>MASTVSNTSKLEKPVSLIWGCELNEQNKTFEFKVEDDEEKCEHQLALRTVCLGDKAKDEFHIVEIVTQEEGAEKSVPIATLKPSILPMATMVGIELTPPVTFRLKAGSGPLYISGQHVAMEEDYSWAEEEDEGEAEGEEEEEEEEDQESPPKAVKRPAATKKAGQAKKKLDKEDESSEEDSPTKKGKGAGRGRKPAAKK[5x]

In Xenopus eggs, NPM2 replaces sperm protamines with core histones upon fertilization, thereby promoting nucleosome assembly on sperm DNA Laskey et al., 1978; Philpott et al., 1991; Ohsumi and Katagiri, 1991. NPM2 can also extract out somatic linker histones from chromatin Dimitrov and Wolffe, 1996; Ramos et al., 2005; Bañuelos et al., 2007. The acidic tracts in the C-terminal tail of NPM2 binds H2A-H2B, histone octamers, and the linker histone H5 Platonova et al., 2011; Ramos et al., 2010; Taneva et al., 2009, while poly-glutamylation and hyperphosphorylation of NPM2 promote its substrate sequestration ; Lorton et al., 2023. Our cryo-EM structure strongly suggests that the NPM2 binds to H1.8 as a homo-pentamer.

By further analyzing our cryo-EM structure representing the H1.8-bound state of NPM2, we identified two structural variants, classified as open and closed forms. The major structural differences between the two forms are found at C-terminal and N-terminal segments of NPM2 core and at the A1 loop. In the open form, however, the C-terminal portion of β8 is bent outward to the rim. Along with this β8 bending, C-terminal segment, N-terminal segment, and A1 loop are also positioned outward in the open form. The bending is critical in forming the open-form NPM2 structures and increases the accessibility of the H1-binding sites. Notably, extra cryo-EM densities, which may represent H1.8, are clearly observed in the open form but much less in the closed form near the acidic surface regions proximal to the N terminus of β1 and the C terminus of β8. Supporting this idea, the acidic tract A1 (aa 36–40) and A2 (aa 120–140), which are both implicated in the recognition of basic substrates such as core histones Dutta et al., 2001; Platonova et al., 2011, respectively interact with and are adjacent to the putative H1.8 density. In addition, the NPM2 surface that is in direct contact with the putative H1.8 density is accessible in the open form while it is internalized in the closed form. Structure variation analyses suggest that NPM2 subunits can exhibit two structural configurations, open and closed forms, of which H1.8 is stably associated with only the open form. As the A2 and A3 belong to the disordered C-terminal tail that extends from the petal side of the NPM2 complex, our data suggest that the open form provides a stable association platform by exposing the acidic surface at the petal side for the substrate recognition, while the C-terminal A2 and A3 at the flexible tail may facilitate recruitment and possibly also entrapment of the substrate.> ANKNMKILIVDDFSTMRRIVKNLLRDLGFNNTQEADDGLTALPMLKKGDFDFVVTDWNMPGMQGIDLLKNIRADEELKHLPVLMITAEAKREAIIEAAQAGVNGYIVKPFTAATLKEKLDKIFE

Vibrio cholerae contains multiple copies of chemotaxis response regulator (VcCheY1–VcCheY4) whose functions are elusive yet. Autophosphorylated CheA then donates phosphate to the response regulator CheY. Phosphorylated CheY interacts with the flagellar motor protein FliM and influence the direction of flagellar rotation from counter clock wise (CCW) to clock wise (CW). As expected, both VcCheY3 and VcCheY4 possess (β/α)5 fold typical of the response regulators.

To investigate whether the hydrogen bond between T90 and Q97 affects the hydrophobic packing of W61, M88 and V106, we have solved the structure of VcCheY3-Q97A. As expected, the overall structure of VcCheY3-Q97A is almost identical to that of VcCheY3 and the Mg2+ ion bound at the active site occupies the equivalent position to that of Mg2+ (or Ca2+) of VcCheY3. Interestingly, even in the absence of the hydrogen bond between T90 and Q97, the conformation and packing of W61, M88 and V106 are found to be unaltered with respect to the wild type VcCheY3. However, the water mediated hydrogen bond between W61 and E100 is not seen in this mutant. E100 is slightly reoriented here and has moved toward the CD1 atom of the adjacent I69. These observations, coupled with the quenching results, point to the fact that although the hydrophobic packing of W61, M88 and V106 is independent of the hydrogen bond between T90 and Q97 in free state, in the absence of the later interaction, reorientation of W61 and M88 occurs more smoothly upon phosphorylation. VcCheY3-Q97A and VcCheY3-Q97A/E100A, on the other hand, showed considerable quenching in the presence of acP, suggesting that in the absence of the hydrogen bond between T90 and Q97 (and also in absence of E100), conformational alteration of W61 may take place more easily and it can move toward the surface of the molecule. Km value, obtained by us, was the highest for VcCheY3 (6.4±0.45 mM) followed by VcCheY3-Q97A (2.3±0.4 mM) and VcCheY3-Q97A/E100A (2.0±0.2 mM) which are in accordance with our structural observations. The lower Km values of VcCheY3-Q97A and VcCheY3-Q97A/E100A are due to the loss of the coupling between T90 and Q97 which facilitates the movement of T90 toward the active site and stabilize the acyl phosphate. Furthermore, aforesaid biochemical data, in conjunction with the structure of VcCheY3-Q97A, indicated that the coupling of T90 and Q97 restricts the movement of T90 toward the active site reducing the stabilization of the bound phosphate and effectively promoting autodephosphorylation of VcCheY3.> GGPNLFVALYDFESRTENTLSITKGEKLRVLGYNHNGEWCEAQTKN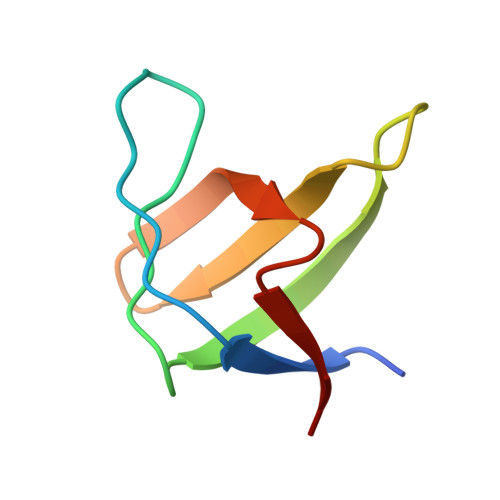GQGWVPSNYITPVN> GSHMASNVLALDTSQRIRIGLRKGEDLFEISYTGEKKHAEILPVVVKKLLDELDLKVKDLDVVGVGIGPGGLTGLRVGIATVVGLVSPYDIPVAPLNSFEMTAKSCPADGVVLVARRAR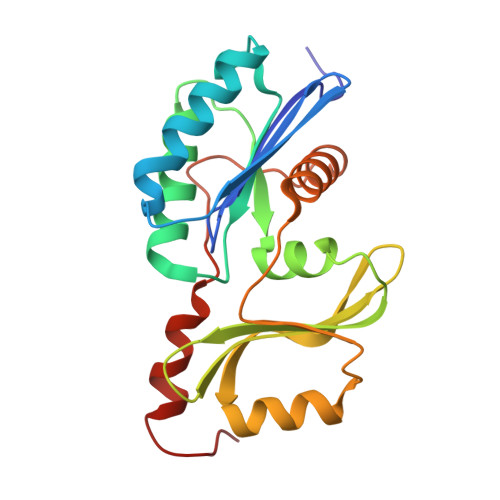KGYHYCAVYLKDKGLNPLKEPSVVSDEELEEITKEFSPKIVLKDDLLISPAVLVEESERLFREKKTIHYYEIEPLYLQKSIAELNWEKKKRG> MSHPIQFVNANNSDKSHQLGGQYSIPQDLRENLQKEAARIGENEKDVLQEKMETRTVQNREDSYHKRRFDMKFEPDSDTQTVTSSENTQDAVVPRKRKSRWDVKGYEPPDESSTAVKENSDSALVNVEGIHDLMFFKPSDHKYFADVISKKPIDELNKDEKKERTLSMLLLKIKNGNTASRRTSMRILTDKAVTFGPEMIFNRLLPILLDRSLEDQERHLMIKTIDRVLYQLGDLTKPYVHKILVVAAPLLIDEDPMVRSTGQEIITNLSTVAGLKTILTVMRPDIENEDEYVRNVTSRAAAVVAKALGVNQLLPFINAACHSRKSWKARHTGIKIVQQIGILLGIGVLNHLTGLMSCIKDCLMDDHVPVRIVTAHTLSTLAENSYPYGIEVFNVVLEPLWKGIRSHRGKVLSSFLKAVGSMIPLMDPEYAGYYTTEAMRIIRREFDSPDDEMKKTILLVLQKCSAVESITPKFLREEIAPEFFQKFWVRRVALDRPLNKVVTYTTVTLAKKLGCSYTIDKLLTPLRDEAEPFRTMAVHAVTRTVNLLGTADLDERLETRLIDALLIAFQEQTNSDSIIFKGFGAVTVSLDIRMKPFLAPIVSTILNHLKHKTPLVRQHAADLCAILIPVIKNCHEFEMLNKLNIILYESLGEVYPEVLGSIINAMYCITSVMDLDKLQPPINQILPTLTPILRNKHRKVEVNTIKFVGLIGKLAPTYAPPKEWMRICFELLELLKSTNKEIRRSANATFGFIAEAIGPHDVLVALLNNLKVQERQLRVCTAVAIGIVAKVCGPYNVLPVIMNEYTTPETNVQNGVLKAMSFMFEYIGNMSKDYIYFITPLLEDALTDRDLVHRQTASNVITHLALNCSGTGHEDAFIHLMNLLIPNIFETSPHAIMRILEGLEALSQALGPGLFMNYIWAGLFHPAKNVRKAFWRVYNNMYVMYQDAMVPFYPVTPDNNEEYIEELDLVL;> MWGGGKMAVVSLSPHTAKMRKLFGQASTTMAYDGLKREAERRTRSDHNITMVAKDDELYLYHLTLKKQTNFVHSCIGHFVDLEAGSKREQSQLCVATETHLELYDTADGELKLIAKFQNLFATITSMKSLDLPHSGSRAKASNWPTFLALTSDSGNLSIVQIIMHAGALRLKTLVNQPLTRTTLRRVSPISYMEIDPNGRCIILSSVEQNKLCFLVDYAQKLRISSPLEIIRPHMVTLDMAVVDVNFNNPCFVTLEIDNAATQLSVHLIFYVLELGLNHIVKKADYLVNPSANFVLSLPDLSRYNITTSLSDNNYDADYDTLFNPFVVIGFENHILVKDMNGFFSLKVEIPKRSITNSRHKNVTIISGIVQKLKNDFFVLLQSNHGDLFKLTVSPDTNDRNRPLVQLSYFDTIQNSHQLHIFKNGYLFALSEMNNNFLFQFEKLGVEKNDFSNVLTSKDPNKSLVFEPSIKLQNLSILSQQLNLNPSIKSQIVSDSPLSIATKHFTNNKIITLTNAVNYSNLISTSLPPNATKLWLIPDPATTGDNNTLLFITFPKKTMILQIDNESMEELTPDEATRSAFKLSQDTTIHTCLMGSHSIIQVCTAELRHIVPTGKSRYSNKLTWVPPAGIRIVCATSSKTQLIISLSNYELVYFKIDVSSDSLIELTTHPELDTMPSKVAIVQDTQHADLLAIADNEGMIKIMSLKDQKEDFLTVISLQLVSEKISDMIMVRDSSIGQLNLHVGLENGVYMKFHIGDVDGSFTDIKRRFLGLKPVSLSYLREISVSLNNEEEEEEEEDDDDEKEEEEINSSGAKWMSCVVCHSSSTWVSYTWKNVWTIRQLKDQNMLSCSKFVNADVAINGVCSISSSGRLNIGRVSNFPTLDNWFHVHESSVNKQENGGGDESNEEEEDEMEEEMEMLQISTFRPRTILSFPNNPKSILFIDNHSGKKQCRISLQIDGECLKFGSSDHLYKILDDIDCVSAAIIDFTRQADHLIICAGDKRLLTYKILVNKDKLSFDIELLHQTEIISPIHAMLKFKNFLLTAMGSTIVLYGLGKKQLLRRSVTQTPVSITKIVSMHQWNYERLAVGDIHESVTLFIWDPAGNVFIPYVDDSVKRHVTVLKFLDEATVIGADRYGNAWTLRSPPECEKIMSNHDPSELSNGAIKYPLDVITLQQKLPNTYDCKFKFQLLNHFFVNDIITDFHILDSLSNSDRPGCIYMGLQGTVGCFIPLLSKGNVFMMGNIENIMAEADDTFYLDYESRKKNNNMRKEDDEEESGSVVLQGRHGIEDEIICEGSCSILGRDHQEYRSYYAPVRKVIDGDLCENFLRLSLNEQEFLAKNLKSVQVEDIIQTINEVRTNYM;> MARTKSRKRSGNNQNKNASVVNNKAEIAAMIDARRLEQKKKGGVTNSKGKTNKVVDAKLEKEFKDVLQRFQVQENDTPKEITKDEKNNHVVIVEKNPVMNRKHTAEDELEDTPSDGIEEHLSARKRRKTEKPSLSQLKSQVPYPQIIEWYDCDARYPGLLASIKCTKNVIPVPSHWQSKKEYLSGRSLLGKRPFELPDIIKKTNIEQMRSTLPQSGLDGQDEKSLKEASRARVQPKMGALDLDYKKLHDVFFKIGANWKPDHLLCFGDVYYENRNLFEETNWKRMVDHKRPGRISQELRAIMNLPEGQLPPWCMKMKDIGLPTGYPDLKIAGLNWDITNLKGDVYGKIIPNHHSRSKKQGRNYFGALISFETPEFENSKEDTQANAENGRQDDKIDDEVEHKLDHFQEDISEVTSAEEKLERNEEESEKQLYTVLK;> MNYSADSGNTVYVGNIDPRITKEQLYELFIQINPVLRIKYPKDKVLQAYQGYAFIEFYNQGDAQYAIKIMNNTVRLYDRLIKVRQVTNSTGTTNLPSNISKDMILPIAKLFIKNLADSIDSDQLVKIFNKFGKLIREPEIFYLSNGKLKCAYVYFEDFEKADLAIKSLNNQLVANNRITVDYAFKENGKGNAKYGDDVDRLLNKEALKHNMLK;> MSRHQFDLIMCLKQPGVQTGLLCEKC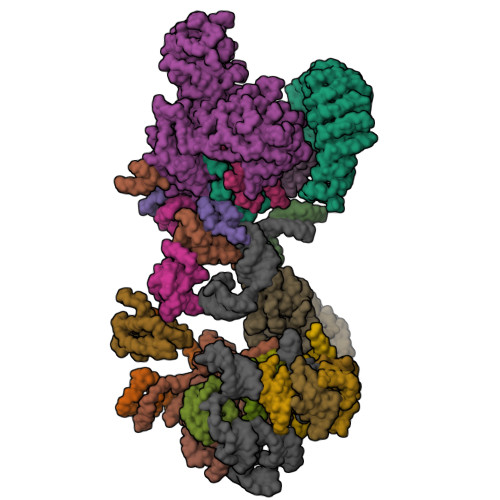DGKCPICDSYVRPKRKVRVCENCSFGKQAKNCIICNLNVGVNDAFYCWECCRLGKDKDGCPRILNLGSNRLDRHFEKKKKV;> MNLLETRRSLLEEMEIIENAIAERIQRNPELYYHYIQESSKVFPDTKLPRSSLIAENKIYKFKKVKRKRKQIILQQHEINIFLRDYQEKQQTFNKINRPEETQEDDKDLPNFERKLQQLEKELKNEDENFELDINSKKDKYALFSSSSDPSRRTNILSDRARDLDLNEIFTRDEQYGEYMELEQFHSLWLNVIKRGDCSLLQFLDILELFLDDEKYLLTPPMDRKNDRYMAFLLKLSKYVETFFFKSYALLDAAAVENLIKSDFEHSYCRGSLRSEAKGIYCPFCSRWFKTSSVFESHLVGKIHKKNESKRRNFVYSEYKLHRYLKYLNDEFSRTRSFVERKLAFTANERMAEMDILTQKYEAPAYDSTEKEGAEQVDGEQRDGQLQEEHLSGKSFDMPLGPDGLPMPYWLYKLHGLDREYRCEICSNKVYNGRRTFERHFNEERHIYHLRCLGIEPSSVFKGITKIKEAQELWKNMQGQSQLTSIAAVPPKPNPSQLKVPTELELEEEDEEGNVMSKKVYDELKKQGLV;> MNYLEGVGSKKGGGGIASESQFNLQRRKEVESLLSKGENVPYTFQDEKDDQVRSNPYIYKNHSGKLVCKLCNTMHMSWSSVERHLGGKKHGLNVLRRGISIEKSSLGREGQTTHDFRQQQKXXXXXXXXXXXXXXXXIIEAKQSLKNNGTIPVCKIATVKNPKNGSVGLAIQVNYSSEVKENSVDSDDKAKVPPLIRIVSGLELSDTKQKGKKFLVIAYEPFENIAIELPPNEILFSENNDMDNNNDGVDELNKKCTFWDAISKLYYVQFFFKQAEQEQADV;> MEPEDTQLKEDIKTTVNYIKQHGVEFENKLLEDERFSFIKKDDPLHEYYTKLMNEPTDTVSGEDNDRKSEREIARPPDFLFSQYDTGISRRDMEVIKLTARYYAKDKSIVEQMISKDGEARLNFMNSSHPLHKTFTDFVAQYKRVYSFTGQEIKKSKRTILDNCFERTQYWEFEKDKDREHDKLVELCKIQFAAIPWDKFTQVAKFSIPEDTEIFEGSLDLEQMRLRRVQTGIKLFDSIKPTNEEEKIVSDQGKQKGGDSKGKKRKIRAVGETRLKKSKK;> MKFTPSIVIDAPQYYVDHFNGKYNVDKCVILRDLQLETDSESMPSSLKHLTKPTHILDLTNNDLIMIPDLSRRDDIHTLLLGRNNIVEVDGRLLPMNVQNLTLSNNSIRRFEDLQRLRRAPRTLKNLTLIGNQVCHLANYREHVLRLVPHLETLDFQNVTAEERKSAMSFPRQADGDTLGPVNTAIRDNGSRDKTMEIMNLVVSKMTVERRNELKKQLAEATSLEEIARLEKLLSGGV;> MVEPARKKQRIDRDTHHTVAEPVTEAKNTLYVSQLNEKINMQRLRVNLFLLFATFGEVLKVSMNFKKQRGQAFITMRTIDQASLAQISLNGERFFGKPLKVEFSKSETKTL;> MAEKQRQLKLQKIYKQKYIGLGDESTTREQWQRNVRNDTLNTLQGHSASLEYVSLSRGDLSIRDTRIHLLKSMSPGYKAYLREE;> METIDSKQNINRESLLEERRKKLAKWKQKKAQFDAQKEHQTSRNDIVTNSLEGKQTTEKFTERQERVKEELRKRKNEFRKSDEPVSVKPSKKKSKRSKVKKKISFDFSDDDDSEIGVSFRSKEHIQKAPEHDNEKDPLDEFMTSLKEEKMSNSKGMYDRGDILDVEDQLFELGGTDDEDVEDNTDNSNIAKIAKLKAKKRVKQIYYSPEELEPFQKNFYIESETVSSMSEMEVEELRLSLDNIKIKGTGCPKPVTKWSQLGLSTDTMVLITEKLHFGSLTPIQSQALPAIMSGRDVIGISKTGSGKTISYLLPLLRQVKAQRPLSKHETGPMGLILAPTRELALQIHEEVTKFTEADTSIRSVCCTGGSEMKKQITDLKRGTEIVVATPGRFIDILTLNDGKLLSTKRITFVVMDEADRLFDLGFEPQITQIMKTVRPDKQCVLFSATFPNKLRSFAVRVLHSPISITINSKGMVNENVKQKFRICHSEDEKFDNLVQLIHERSEFFDEVQSENDGQSSDVEEVDAKAIIFVSSQNICDFISKKLLNAGIVTCAIHAGKPYQERLMNLEKFKREKNSILLCTEVLSRGLNVPEVSLVIIYNAVKTFAQYVHTTGRTARGSRSGTAITLLLHDELSGAYILSKAMRDEEIKALDPLQAKELQEMSAKFESGMKKGKFRLSKGFGGKGLENIKSKREEAQNKDLELKKNDKRSDDLEKKISNPREGHDSVSESSALIPRLNYELFKESTDGSIIFYAKVYINDLPQIVRWEATKNTTLLFIKHETGCSITNKGKFYPEGKEPKNENDEPKLYLLIEGQDEKDIQLSIELLEQKVKEGVVKAASLSLKSTKY;> MSKIQVAHSSRLANLIDYKLRVLTQDGRVYIGQLMAFDKHMNLVLNECIEERVPKTQLDKLRPRKDSKDGTTLNIKVEKRVLGLTILRGEQILSTVVEDKPLLSKKERLVRDKKEKKQAQKQTKLRKEKEKKPGKIAKPNTANAKHTSSNSREIAQPSSSRYNGGNDNIGANRSRFNNEAPPQTRKFQPPPGFKRK;> MKLVNFLKKLRNEQVTIELKNGTTVWGTLQSVSPQMNAILTDVKLTLPQPRLNKLNSNGIAMASLYLTGGQQPTASDNIASLQYINIRGNTIRQIILPDSLNLDSLLVDQKQLNSLRRSGQIANDPSKKRRRDFGAPANKRPRRGL;> MSSQIIDRPKHELSRAELEELEEFEFKHGPMSLINDAMVTRTPVIISLRNNHKIIARVKAFDRHCNMVLENVKELWTEKKGKNVINRERFISKLFLRGDSVIVVLKTPVE;> MTMNGIPVKLLNEAQGHIVSLELTTGATYRGKLVESEDSMNVQLRDVIATEPQGAVTHMDQIFVRGSQIKFIVVPDLLKNAPLFKKNSSRPMPPIRGPKRR;> MSNKVKTKAMVPPINCIFNFLQQQTPVTIWLFEQIGIRIKGKIVGFDEFMNVVIDEAVEIPVNSADGKEDVEKGTPLGKILLKGDNITLITSA;> MSESSDISAMQPVNPKPFLKGLVNHRVGVKLKFNSTEYRGTLVSTDNYFNLQLNEAEEFVAGVSHGTLGEIFIRCNNVLYIRELPN;> MVSTPELKKYMDKKILLNINGSRKVAGILRGYDIFLNVVLDDAMEINGEDPANNHQLGLQTVIRGNSIISLEALDAI>[2x]RHMELSPDGNLKTTITIGDRLTYDITCNGRQILTPSPISMTLDNGTVWGENAKLSGTSRKSVDEMIPSPFYRASELRNHYNGLTLRFKKDWNVEFRAYNDGIAYRFVNQGKKPFRVVTEVSDYCFPSDMTASVPYVKSGKDGDYNSQFFNSFENTYTTDKLSKLNKQRLMFLPLVVDAGDGVKVCITESDLENYPGLYLSASEGANRLSSMHAPYPKRTVQGGHNQLQMLVKEHEDYIAKVDKPRNFPWRIAVVTTTDKDLAATNLSYLLGAPSRMSDLSWIKPGKVAWDWWNDWNLDGVDFVTGVNNPTYKAYIDFASANGIEYVILDEGWAVN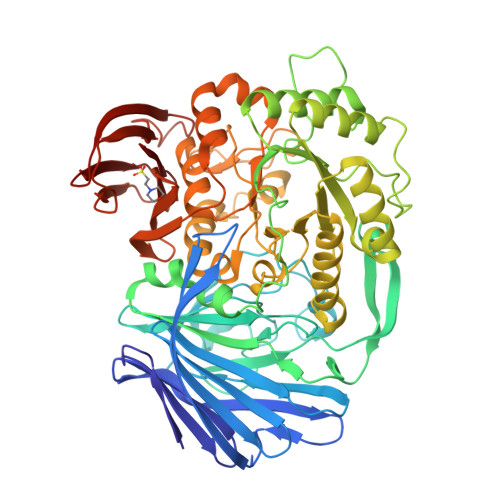LQADLMQVVKEIDLKELVDYAASKNVGIILWAGYHAFERDMENVCRHYAEMGVKGFKVDFMDRDDQEMTAFNYRAAEMCAKYKLILDLHGTHKPAGLNRTYPNVLNFEGVNGLEQMKWSSPSVDQVKYDVMIPFIRQVSGPMDYTQGAMRNASKGNYYPCYSEPMSQGTRCRQLALYVVFESPFNMLCDTPSNYMREPESTAFIAEIPTVWDESIVLDGKMGEYIVTARRKGDVWYVGGITDWSARDIEVDCSFLGDKSYHATLFKDGVNAHRAGRDYKCESFPIKKDGKLKVHLAPGGGFALKIK>[2x]MAIVVDDSVFSPSYVPKRLPHREQQLQQLDILLGNWLRNPGHHYPRATLLGRPGTGKTVTLRKLWELYKDKTTARFVYINGFIYRNFTAIIGEIARSLNIPFPRRGLSRDEFLALLVEHLRERDLYMFLVLDDAFNLAPDILSTFIRLGQEADKLGAFRIALVIVGHNDAVLNNLDPSTRGIMGKYVIRFSPYTKDQIFDILLDRAKAGLAEGSYSEDI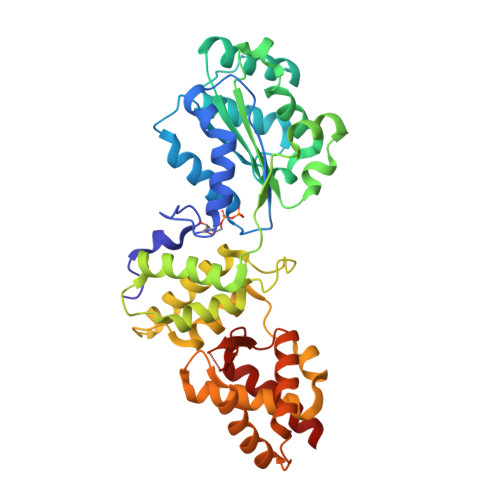LQMIADITGAQTPLDTNRGDARLAIDILYRSAYAAQQNGRKHIAPEDVRKSSKEVLFGISEEVLIGLPLHEKLFLLAIVRSLKISHTPYITFGDAEESYKIVCEEYGERPRVHSQLWSYLNDLREKGIVETRQNKRGEGVRGRTTLISIGTEPLDTLEAVITKLIKEELR>MSKPKQPPDASPANLLTSLVRAHLDSGPSTAKLDYSKFQELVLPHFGKEDAGDVQQFYDLLS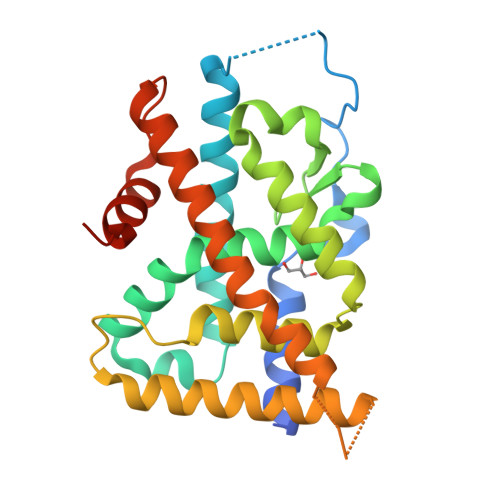GSLEVIRKWAEKIPGFAELSPADQDLLLESAFLELFILRLAYRSKPGEGKLIFCSGLVLHRLQCARGFGDWIDSILAFSRSLHSLLVDVPAFACLSALVLITDRHGLQEPRRVEELQNRIASCLKEHVAAVAGEPQPASCLSRLLGKLPELRTLCTQGLQRIFYLKLEDLVPPPPIIDKIFMDTLPFLEHHHHHH[2x]>[3x]MIQGVIQKIAGPAVIAKGMLGARMYDICKVGEEGLVGEIIRLDGDTAFVQVYEDTSGLKVGEPVVSTGLPLAVELGPGMLNGIYDGIQRPLERIREKTGIYITRGVVVHALDREKKWAWTPMVKPGDEVRGGMVLGTVPEFGFTHKILVPPDVRGRVKEVKPAGEYTVEEPVVVLEDGTELKMYHTWPVR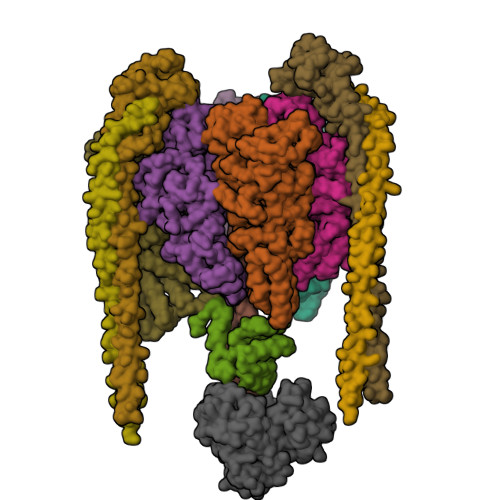RARPVQRKLDPNTPFLTGMRILDVLFPVAMGGTAAIPGPFGSGKTVTQQSLAKWSNADVVVYVGCGERGNEMTDVLVEFPELTDPKTGGPLMHRTVLIANTSNMPVAAREASIYVGVTIAEYFRDQGFSVALMADSTSRWAEALREISSRLEEMPAEEGYPPYLAARLAAFYERAGKVITLGGEEGAVTIVGAVSPPGGDMSEPVTQSTLRIVGAFWRLDASLAFRRHFPAINWNGSYSLFTSALDPWYRENVAEDYPELRDAISELLQREAGLQEIVQLVGPDALQDAERLVIEVGRIIREDFLQQNAYHEVDAYCSMKKAYGIMKMILAFYKEAEAAIKRGVSIDEILQLPVLERIGRARYVSEEEFPAYFEEAMKEIQGAFKALA;>MDLLKKEYTGITYISGPLLFVENAKDLAYGAIVDIKDGTGRVRGGQVIEVSEEYAVIQVFEETTGLDLATTSVSLVEDVARLGVSKEMLGRRFNGIGKPIDGLPPITPEKRLPITGLPLNPVARRKPEQFIQTGISTIDVMNTLVRGQKLPIFSGSGLPANEIAAQIARQATVRPDLSGEGEKEEPFAVVFAAMGITQRELSYFIQEFERTGALSRSVLFLNKADDPTIERILTPRMALTVAEYLAFEHDYHVLVILTDMTNYCEALREIGAAREEIPGRRGYPGYMYTDLATIYERAGVVEGKKGSVTQIPILSMPDDDRTHPIPDLTGYITEGQIQLSRELHRKGIYPPIDPLPSLSRLMNNGVGKGKTREDHKQVSDQLYSAYANGVDIRKLVAIIGEDALTENDRRYLQFADAFERFFINQGQQNRSIEESLQIAWALLSMLPQGELKRISKDHIGKYYGQKLEEIWGAPQALD[3x];> MSQVSPTRMNLLQRRGQLRLAQKGVDLLKKKRDALVAEFFGLVREAMEARKALDQAAKEAYAALLLAQAFDGPEVVAGAALGVPPLEGVEAEVENVWGSKVPRLKATFPDGALLSPVGTPAYTLEASRAFRRYAEALIRVANTETRLKKIGEEIKKTTRRVNALEQVVIPGIRAQIRFIQQVLEQREREDTFRLKRIKGKIEAREAEEEGGRPNPQVEIGAGL;> MAVIADPETAQGFRLAGLEGYGASSAEEAQSLLETLVERGGYALVAVDEALLPDPERAVERLMRGRDLPVLLPIAGLKEAFQGHDVEGYMRELVRKTIGFDIKL;>GGGLGLIKSLAEKEKQLLERLEAAKKEAEERVKRAEAEAKALLEEAEAKAKALEAQYRERERAETEALLARYRERAEAEAKAVREKAMARLDEAVALVLKEVLP[2x];>[2x]MSKLEAILSQEVEAEIQALLQEAEAKAEAVKREAEEKAKALLQARERALEAQYRAALRRAESAGELLVATARTQARGEVLEEVRRRVREALEALPQKPEWPEVVRKLALEALEALPGAKALVANPEDLPHLEAMARERGVELQAEPALRLGVRAVGAEGKTQVENSLLARMDRAWDAMSSKVAQALWG;> MADDFAYLNARVRVRRGTLLKESFFQEALDLSFADFLRLLSETVYGGELAGQGLPDVDRAVLRTQAKLVGDLPRLVTGEAREAVRLLLLRNDLHNLQALLRAKATGRPFEEVLLLPGTLREEVWRQAYEAQDPAGMAQVLAVPGHPLARALRAVLRETQDLARVEALLAKRFFEDVAKAAKGLDQPALRDYLALEVDAENLRTAFKLQGSGLAPDAFFLKGGRFVDRVRFARLMEGDYAVLDELSGTPFSGLSGVRDLKALERGLRCVLLKEAKKGVQDPLGVGLVLAYVKEREWEAVRLRLLARRAYFGLPRAQVEEEVVCP>[2x]GAHMDCHLSDMLQQLHSVNASKPSERGLVRQEEAEDPACIPIFWVSKWVDYSDKYGLGYQLCDNSVGVLFNDSTRLILYNDGDSLQYIERDGTESYLTVSSHPNSLMKKITLLKYFRN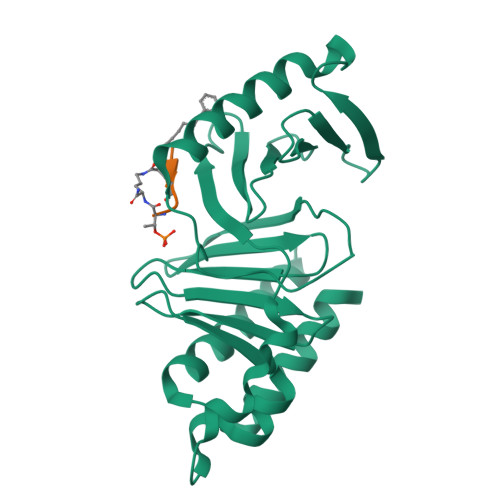YMSEHLLKAGANITPREGDELARLPYLRTWFRTRSAIILHLSNGSVQINFFQDHTKLILCPLMAAVTYIDEKRDFRTYRLSLLEEYGCCKELASRLRYARTMVDKLLSSRSASNRLKAS;>[2x]XPLAST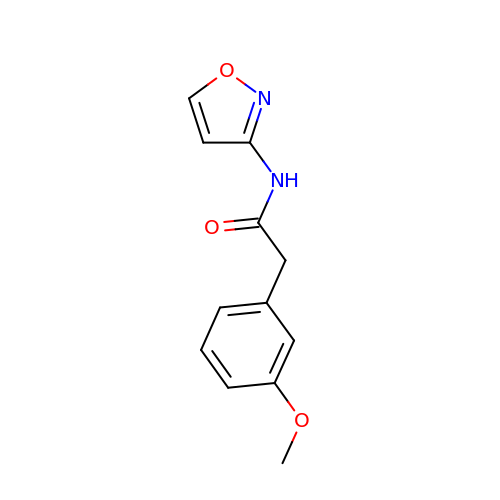2-(3-methoxyphenyl)-N-(1,2-oxazol-3-yl)acetamide | C12 H12 N2 O3 | LFZVRGLOBRIGDU-UHFFFAOYSA-N>[2x]ARTFFVGGNFKLNGSKQSIKEIVERLNTASIPENV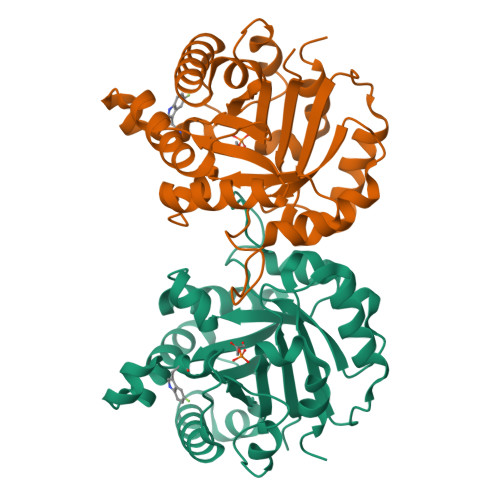EVVICPPATYLDYSVSLVKKPQVTVGAQNAYLKASGAFTGENSVDQIKDVGAKYVILGHSERRSYFHEDDKFIADKTKFALGQGVGVILCIGETLEEKKAGKTLDVVERQLNAVLEEVKDFTNVVVAYEPVWAIGTGLAATPEDAQDIHASIRKFLASKLGDKAASELRILYGGSANGSNAVTFKDKADVDGFLVGGASLKPEFVDIINSRN>[36x]MLGSGFKAERLRVNLRLVINRLKLLEKKKTELAQKARKEIADYLAAGKDE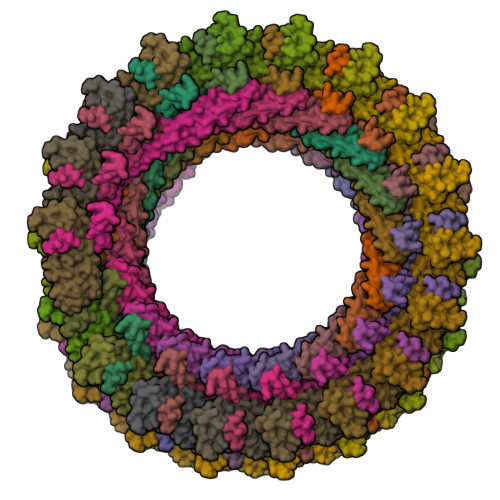RARIRVEHIIREDYLVEAMEILELYCDLLLARFGLIQSMKELDSGLAESVSTLIWAAPRLQSEVAELKIVADQLCAKYSKEYGKLCRTNQIGTVNDRLMHKLSVEAPPKILVERYLIEIAKNYNVPYEPDSVVMAEAPP;>MSNMEKHLFNLKFAAKELSRSAKKCDKEEKAEKAKIEKAIQKGNMEVARIHAENAIRQKNQAVNFLRMSARVDAVAARVQTAVTMGKVTKSMAGVVKSMDATLKTMNLEKISALMDKFEHQFETLDVQTQQMEDTMSSTTTLTTPQNQVDMLLQEMADEAGLDLNMELPQGQTGSVGTSVASAEQDELSQRLARLRDQV[36x]> ATTLKEAADGAGRDFGFALDPNRLSEAQYKAIADSEFNLVVAENAMKWDATEPSQNSFSFGAGDRVASYAADTGKELYGHTLVWHSQLPDWAKNLNGSAFESAMVNHVTKVADHFEGKVASWDVVNAAFADGGGRRQDSAFQQKLGNGYIETAFRAARAADPTAKLCINDYNVEGINAKSNSLYDLVKDFKARGVPLDCVGFQSNLIVGQVPGDFRQNLQRFADLGVDVRITELDIRMRTPSDATKLATQAADYKKVVQACMQVTRCQGVTVWGITDKYSWVPDV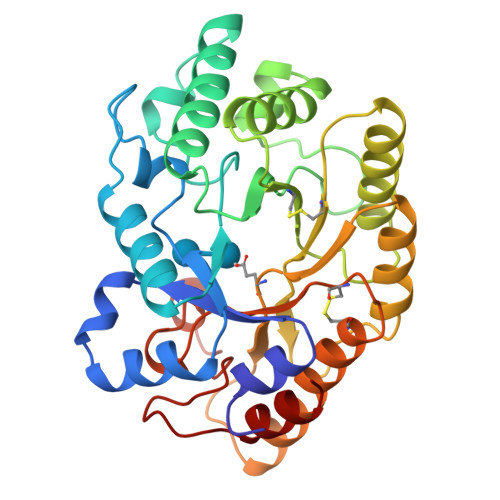FPGEGAALVWDASYAKKPAYAAVMEAF>MGSHQERPLIGLLFSETGVTADIERSQRYGALLAVE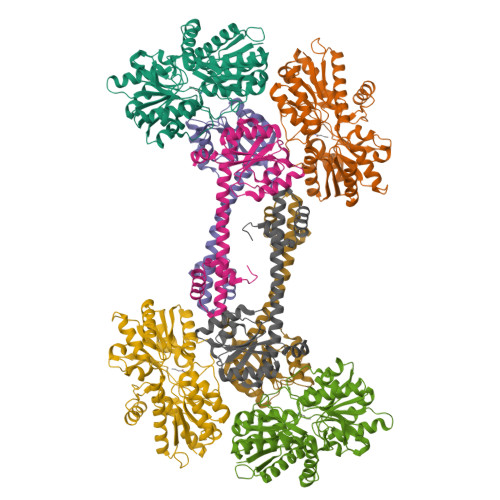QLNREGGVGGRPIETLSQDPGGDPDRYRLCAEDFIRNRGVRFLVGCYMSHTRKAVMPVVERADALLCYPTPYEGFEYSPNIVYGGPAPNQNSAPLAAYLIRHYGERVVFIGSDYIYPRESNHVMRHLYRQHGGTVLEEIYIPLYPSDDDLQRAVERIYQARADVVFSTVVGTGTAELYRAIARRYGDGRRPPIASLTTSEAEVAKMESDVAEGQVVVAPYFSSIDTPASRAFVQACHGFFPENATITAWAEAAYWQTLLLGRAAQAAGNWRVEDVQRHLYDIDIDAPQGPVRVERQNNHSRLSSRIAEIDARGVFQVRWQSPEPIRPDPYVVVHNLDDWSASMGGGPLP[2x];>MSANSLLGSLRELQVLVLNPPGEVSDALVLQLIRIGCSVRQCWPPPEAFDVPVDVVFTSIFQNRHHDEIAALLAAGTPRTTLVALVEYESPAVLSQIIELECHGVITQPLDAHRVLPVLVSARRISEEMAKLKQKTEQLQDRIAGQARINQAKVLLMQRHGWDEREAHQHLSREAMKRREPILKIAQELLGNEPSA[2x]>[2x]MMQFTMSGTMLRFDETTLRFSFSRDGATWSGCDGIEPQLTREDRSFSFAGAATVTHERIETGTGVGVRSVFAGFAGADYAFETYIWIERSSGDVLCEWVPLRECGAEPRIDRVLWPAPLSFDRADAHDVTLITHEQGVMIPNSWPTEVGTDAVSFGGRFETAGGYMPWFAQLRSDGHAYIAICETPWNAGYDIDHPAGGPYTHVGMWFEPSLGRMDYRRVVRYRLLDHADHTAICKTYRAYVNERGRLRTLAEKAARNPSVRDLLGRSWVHVGIKTNVQPDSSFYDPAQPGKNDSLVTFAQRERQMRTLHEMGAGRLYLHLDGWAQPGYDNGHPDYLPACREAGGWKGMKSLIDACHEQGDLFGTHDQYRDYYFAARTFDPRNAIRLADGTMPEHAMWAGGRQTYLCAELAPDYVRRNFSEIATHGIVLDCAYLDVFTCNEGDECSHPEHRMTRRECYERR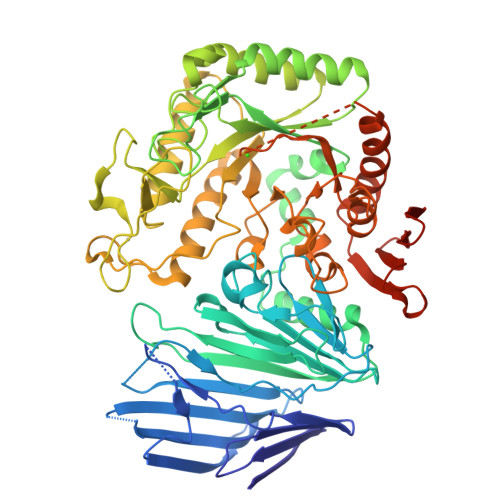AECFEYLLAHGILTSSEEVSDWAVPSLVFCHYAPYDFQMRSPDAPRHGIPVPLYNLVYHDCVIQPWMMDRVAGGDDYMLYALLNGGAPYLIRDAAYAGMDGDMNAALRARTENDIERCAVVAGLHRRVGMQELVRHDLVGGDPLVQRSVFADGTAVTCDFHAQTYEVAANGSHHHHHHH>[2x]MHHHHHHASDYKDDDDKGSLVPRGSPLLDDDDQVAFSFILDNIVTQKMMAVPDSWPFHHPVNKKFVPDYYKVIVNPMDLE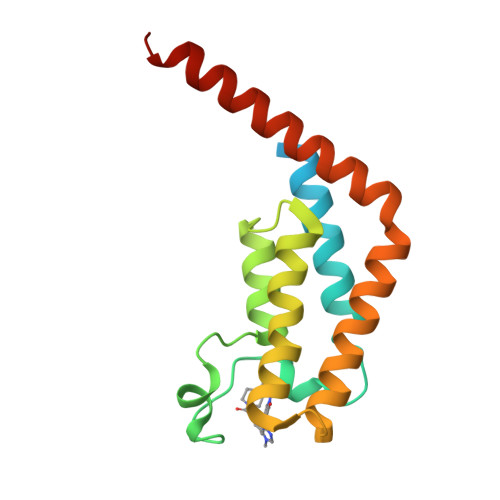TIRKNISKHKYQSRESFLDDVNLILANSVKYNGPESQYTKTAQEIVNVCYQTLTEYDEHLTQLEKDICTAKEAALEEAELESLDPMT MnmE is an evolutionary conserved G protein found in bacteria, fungi, and humans, which together with the protein GidA catalyzes the formation of a carboxymethylaminomethyl-group (cmnm) at the 5 position of the wobble uridine (U34) of tRNAs reading 2-fold degenerated codons ending with A or G, i.e., tRNAArg(UCU), tRNAGln(UUG), tRNAGlu(UUC), tRNALeu(UAA), and tRNALys(UUU). The crystal structure of MnmE from Thermotoga maritima reveals a three-domain protein consisting of an N-terminal tetrahydrofolate-binding domain, a central helical domain, and a canonical Ras-like G domain inserted into the helical domain. On the basis of the common feature that the G domain cycle is regulated by homodimerization, MnmE has been categorized as G protein activated by nucleotide-dependent dimerization (GAD), together with the signal recognition particle (SRP) and its receptor (SR), the regulator of Ni insertion into hydrogenases HypB, the dynamins, the human guanylate binding protein hGBP1, the chloroplast import receptors Toc33/34, the septins, and the Roc-COR tandem found to be mutated in Parkinson disease. The X-ray structures show MnmE to be a constitutive homodimer where the highly mobile G domains face each other in various orientations but are not in close contact as suggested by the GDP-AlFx structure of the isolated domains.

In the case of CtMnmE·GppCp, the crystallographic asymmetric unit contained three protomers (chains A, B, C). Molecules B and C form a dimer within the asymmetric unit, while protomer A forms a dimer with its crystallographic symmetry mate. No density is found for the G domain of molecule C, but crystals applied on an SDS-page confirmed an intact protein (unpublished data). Thus two dimeric structures of CtMnmE·GppCp were analyzed, i.e., the dimer generated by protomer A and a symmetry related chain A (termed “dimer A”) and the dimer generated by protomer B and a second protomer B docked onto chain C (termed “dimer B”). Crystal contacts of G domains A and B in the CtMnmE·GppCp structure comprise areas of 845 Å2 and 987 Å2, respectively. Docking the G domain of molecule B (or A) into the asymmetric unit of the CtMnmE·GppCp structure to the position expected for the G domain of molecule C would create a much smaller hypothetical crystal contact area of only 18 Å2 (or 131 Å2). Thus we would expect that the G domain of molecule C is present in the crystal but, due to its high mobility and absence of sufficient crystal contacts, is not visible in the electron density map. In the crystal structure of CtMnmE·GppCp this loop region is not resolved underlining its high flexibility. In the crystal structure of GppCp-bound MnmE the G domains are found in the open state, indicating that this equilibrium is shifted towards the open state under the crystallization conditions. Moreover, for CtMnmE we find different orientations between the GDP- and GppCp-bound structures and even between different molecules in one asymmetric unit of CtMnmE·GppCp.

>GSHMSPSDLHLPVPGHPIAAIATPVGVGALAIVRISGAGVLDLADRVFRKVHGSGKLAEAAGYTAHFGRLYDGEEMVDEVIALVFRAPRSFTAEQMVEFTCHGGPVVVGRVLRLMLDNGCRLAEPGEFTRRAFLNGRIDLLQAEAIGEMIHARTESAYRTAVSQMKGDLSVRLGGLREQLIRSCALIELELDFSEEDVEFQSRDELTMQIETLRSEVNRLIDSYQHGRIVSEGVSTVIAGKPNAGKSTLLNTLLGQERAIVSHMPGTTRDYIEECFIHDKTMFRLTDTAGLREAGEEIEHEGIRRSRMKMAEADLILYLLDLGTERLDDELTEIRELKAAHPAAKFLTVANKLDRAANADALIRAIADGTGTEVIGISALNGDGIDTLKQHMGDLVKNLDKLHEASVLVTSLRHYEALRNASDALQNALELIAHESETELIAFELRAALDYVGQITGKVVNEEVLNTIFDKFCIGK[3x]>GSHMDDALRGELASALDTEGHALPFDVHLQQPHSSGDGTAGDTSTIQLEKLSHPPARFDLLTNSFVYKWQTKAALARKVSGPMREWAAELKYRTGVHIELEPTYPERLSENAVKGSGSDDGDGTQWGAYETADDVDITVYLFGSERGIFNCHKLMEAAIQQDPVYVRLGIFRRLANSSEVEWLMLRRINRELRPPDIPPISLKLPGKWTLLYERYKEAAIRTLWEETGITVDASNVYPTGHLYQTVPQYYWRVPVRYFVAEVPSDIRVEGPQVVPLQYMRNWDARLLRQSPDPIDRAWAQLADPATGCAWMKASMIDQLQKPLRGDNYMAI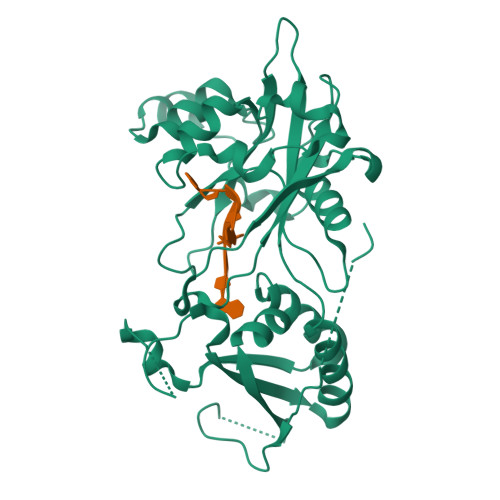RYTPPPYSNLQEVVGLGDGSITPSTGNGEDAS[2x]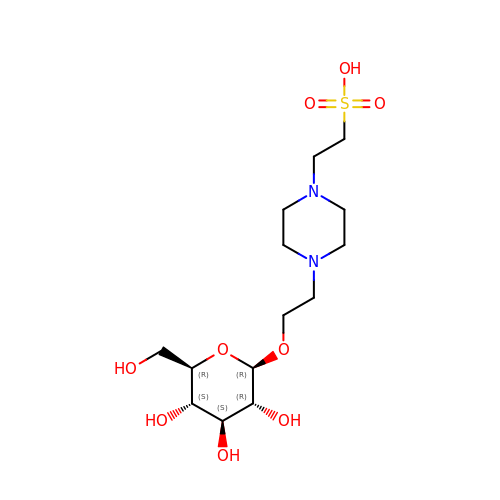2-{4-[2-(beta-D-glucopyranosyloxy)ethyl]piperazin-1-yl}ethanesulfonic acid | C14 H28 N2 O9 S | RRNQQJMHWBFGHX-RKQHYHRCSA-N>[2x]MASGSVLTAIDNDKVAVGDKVTLTINVDKITNFSGYQFNIKYNTTYLQPWDTIADEAYTDSTMPDYGTLLQGRFNATDMSKHNLSQGVLNFGRLYMNLSAYRASGKPESTGAVAKVTFKVIKEIPAEGIKLATFENGSSMNNAV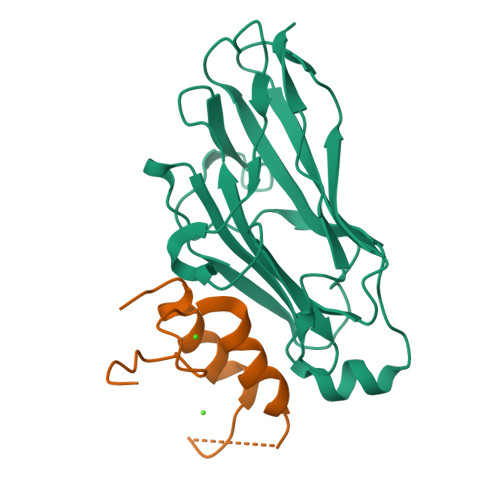DGTMLFDWDGNMYSSSAYKVVQPGLIYPKLEHHHHHH;>[2x]MFVKLKGDLNGDGVINMADVMILAQSFGKAIGNPGVNEKADLNNDGVINSDDAIILAQYFGKTKSAEVVMF>SNAMAEDKGRKVVVSALQFACTDDVSTNVTTAERLVRAAHKQGANIVLIQELFEGYYFCQAQREDFIQRAKPYKDHPTIMRLQKLAKELGVVIPVSFFEEANNAHYNSIAIIDADGTDLGIYRKSHIPDGPGYEEKFYFNPGDTGFKVFQTKYAKIGVAISWDQWFPEAARAMALQGAEILFYPTAIGSEPHDQSIDSRDHWKRVMQGH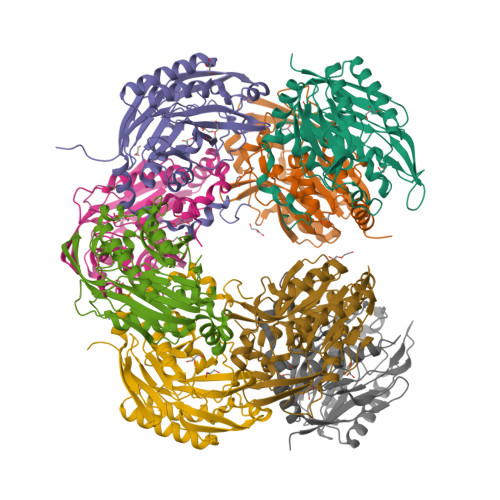AGANLVPLVASNRIGNEIIETEHGKSEIKFYGNSFIAGPTGEIVSIADDKEEAVLIAEFNLDKIKSMRHCWGVFRDRRPDLYKVLLTLDGKNPVL[16x]[(5~{R})-2-[[3,5-bis(fluoranyl)-4-[[3-(trifluoromethyl)-1~{H}-pyrrolo[2,3-b]pyridin-4-yl]oxy]phenyl]amino]-5-fluoranyl-4,6-dihydro-1,3-oxazin-5-yl]methanol | C19 H14 F6 N4 O3 | 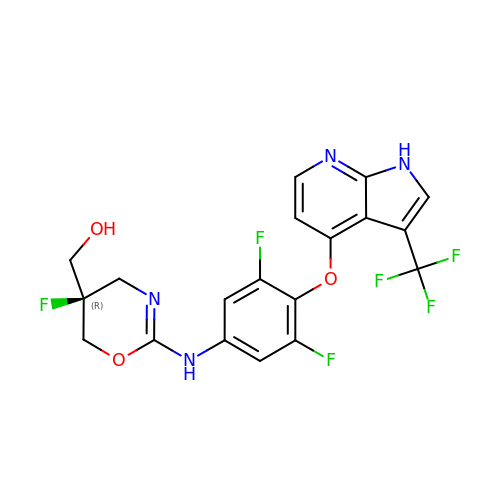PYDVLJUXRPAWOU-GOSISDBHSA-N>[2x]SELNEKLATAWEGFTKGDWQNEVNVRDFIQKNYTPYEGDESFLAGATEATTTLWDKVMEGVKLENRTHAPVDFDTAVASTITSHDAGYINKQLEKIVGLQTEAPLKRALIPFGGIKMIEGSCKAYNRELDPMIKKIFTEYRKTHNQGVFDVYTPDILRCRKSGVLTGLPDAYGRGRIIGDYRRVALYGIDYLMKDKLAQFTSLQADLENGVNLEQTIRLREEIAEQHRALGQMKEMAAK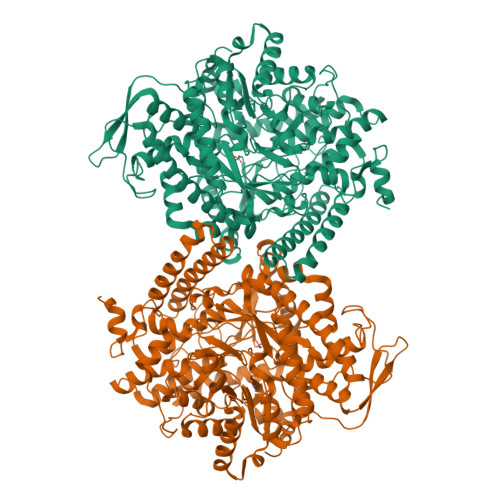YGYDISGPATNAQEAIQWTYFGYLAAVKSQNGAAMSFGRTSTFLDVYIERDLKAGKITEQEAQEMVDHLVMKLRMVRFLRTPEYDELFSGDPIWATESIGGMGLDGRTLVTKNSFRFLNTLYTMGPSPEPNMTILWSEKLPLNFKKFAAKVSIDTSSLQYENDDLMRPDFNNDDYAIAAAVSPMIVGKQMQFFGARANLAKTMLYAINGGVDEKLKMQVGPKSEPIKGDVLNYDEVMERMDHFMDWLAKQYITALNIIHYMHDKYSYEASLMALHDRDVIRTMACGIAGLSVAADSLSAIKYAKVKPIRDEDGLAIDFEIEGEYPQFGNNDPRVDDLAVDLVERFMKKIQKLHTYRDAIPTQSVLTITSNVVYGKKTGNTPDGRRAGAPFGPGANPMHGRDQKGAVASLTSVAKLPFAYAKDGISYTFSIVPNALGKDDEVRKTNLAGLMDGYFHHEASIEGGQHLNVNVMNREMLLDAMENPEKYPQLTIRVSGYAVRFNSLTKEQQQDVITRTFTQSM>[2x]DDLSGFKKIKLGELELFILTDGYIHEENLISFAPRGNVAELKTILKDNFRADHYIDMAINILLVKTKEKLILMDTGMGIFADERTGFLLKSLQKAGFSAHDI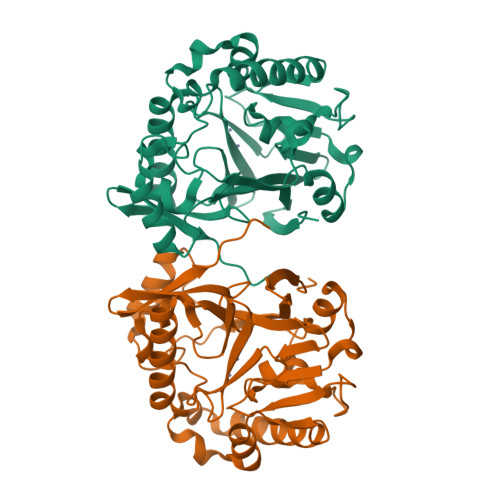TDIFLSHAHPDHIGGVVDKQNKLVFPNASIFISKIEHDFWINASIKDFNNSALKAHPERLNQIIPALQNILKAIQPKLKFYDLNKTLYSHFNFQLAPGHTPGLTVTTISSGNEKLMYVADLIHSDVILFPHPDWGFSGDTDLDIATASRKKFLKQLADTKARAFTSHLPWPGLGFTKVKAPGFEWIPESFMN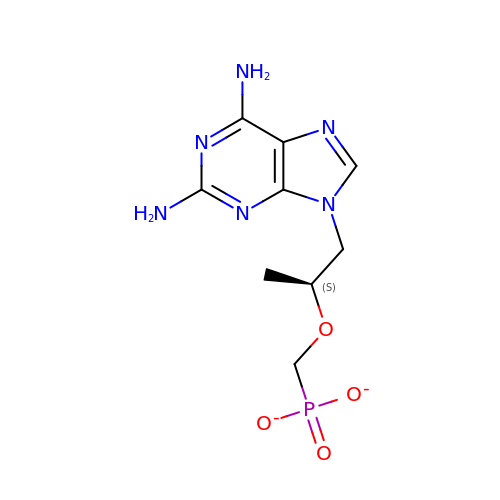2,6-DIAMINO-(S)-9-[2-(PHOSPHONOMETHOXY)PROPYL]PURINE | C9 H13 N6 O4 P | LWEKFDHXJHJYGB-YFKPBYRVSA-L> GSHMAGAQDFVPHTADLAELAAAAGECRGCGLYRDATQAVFGAGGRSARIMMIGEQPGDKEDLAGLPFVGPAGRLLDRALEAADIDRDALYV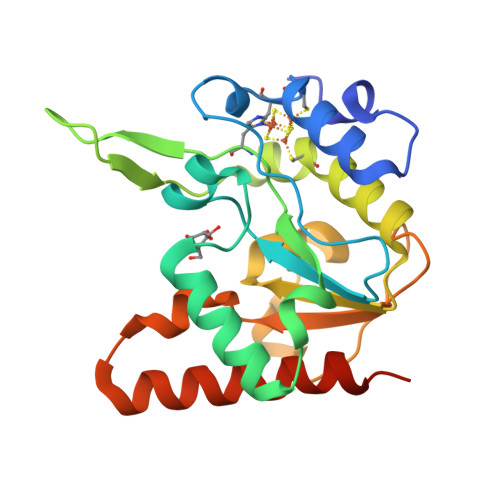TNAVKHFKFTRAAGGKRRIEKTPSRTEVVACRPWLIAEMTSVEPDVVVLLGATAAKALLGNDFRVTQHRGEVLHVDDVPGDPALVATVHPSSLLRGPKEERESAFAGLVDDLRVAADVRPQACGRTR>MPLPTFPALLFGLSGCLVDFGAQAATSDTPDDEHAQLTPGAQNALKALRDQGMPCAWIDELPEALSTPLAAPVNDWMIAAPRPTAGWPQPDACWMALMALNVSQLEGCVLISGDPRLL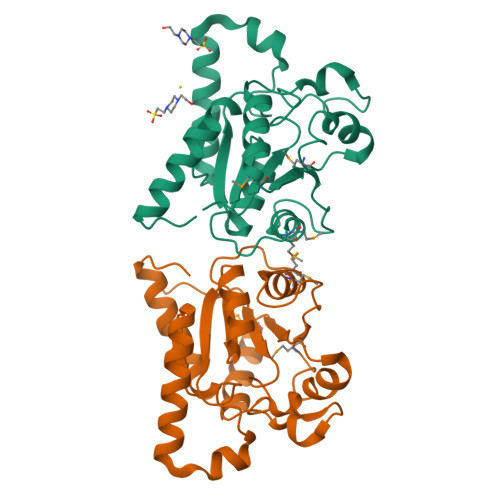QSGLNAGLWTIGLASCGPLCGLSPSQWQALNNAEREQRRAQATLKLYSLGVHSVIDHLGELESCLADIALRRSKGEKP[2x]>SNVPHKSSLPEGIAPGTVLAIRGLVPPNASRFHVNL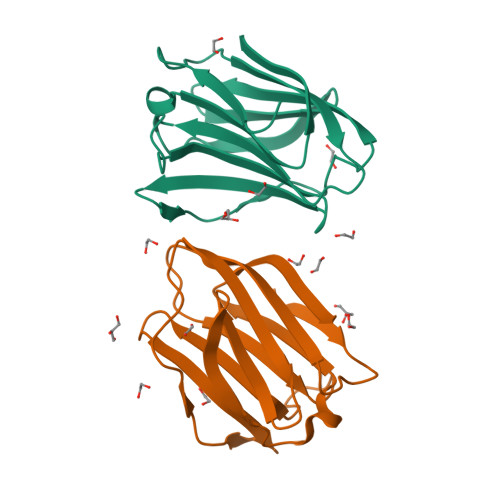LCGEEQGSDAALHFNPRLDTSEVVFNSKEQGSWGREERGPGVPFQRGQPFEVLIIASDDGFKAVVGDAQYHHFRHRLPLARVRLVEVGGDVQLDSVRIF[4x]>[2x]KVQLKGRDLLTLKNFTGEEIKYMLWLSADLKFRIKQ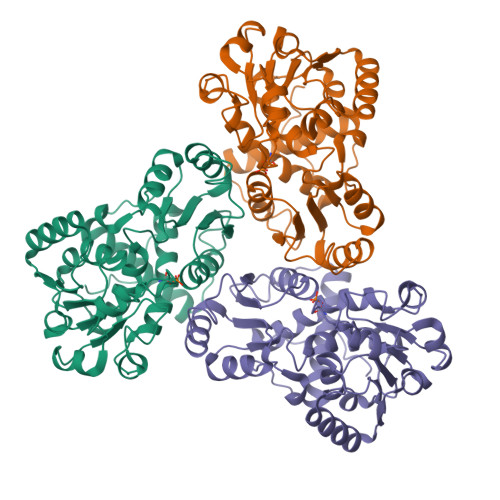KGEYLPLLQGKSLGMIFEKRSTRTRLSTETGFALLGGHPCFLTTQDIHLGVNESLTDTARVLSSMADAVLARVYKQSDLDTLAKEASIPIINGLSDLYHPIQILADYLTLQEHYSSLKGLTLSWIGDGNNILHSIMMSAAKFGMHLQAATPKGYEPDASVTKLAEQYAKENGTKLLLTNDPLEAAHGGNVLITDTWISMGREEEKKKRLQAFQGYQVTMKTAKVAASDWTFLHCLPRKPEEVDDEVFYSPRSLVFPEAENRKWTIMAVMVSLLTDYSPQLQKPKF>[2x]KKSQYLEKINEVIRRAWAVPTHGHELGYSLCNSLRQSGGLDLLMKNCVKPDLQFSSAQLLEQCLTTENRKHVVDNGLDKVVNVACVCTKNSNMEHSRVGTGILEHLFKHSEGTCSDVIRLGGLDAVLFECRTSDLETLRHCASALANLSLYGGAENQEEMILRKVPMWLFPLAFHNDDNIKYYACLAIAVLVANKEIEAEVLKSGCLDLVEPFVTSHDPSAFARSNLAH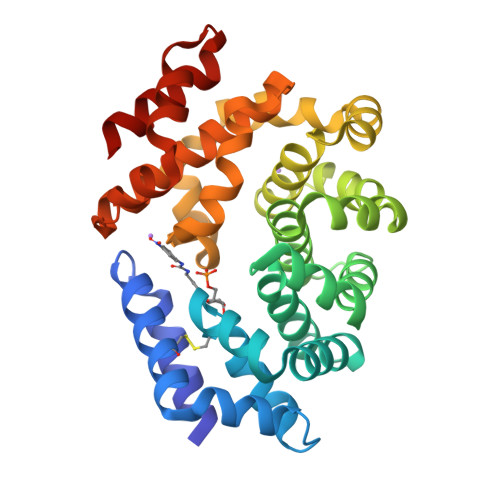AHGQSKHWLKRLVPVLSSNREEARNLAAFHFCMEAGIKREQGNTDIFREINAIEALKNVASCPNAIASKFAAQALRLIGET(S)-4-AMINO-4-OXO-3-(2-PHOSPHONOACETAMIDO)BUTANOIC ACID | C6 H11 N2 O7 P | 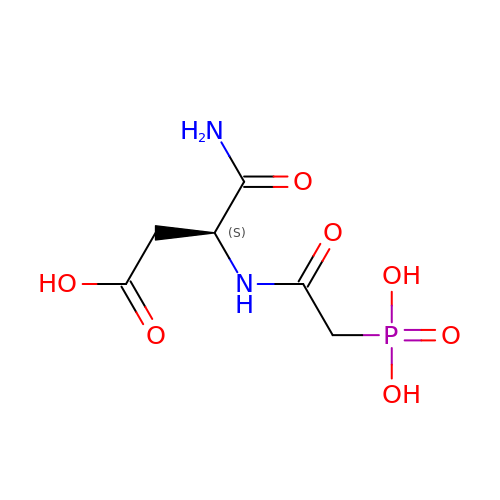HCFYWDYKLQITSR-VKHMYHEASA-N> VQEGQKIDLPKKRYYRQRAHSNPFSDHQLEYPVSPQDMDWSKLYPYYKNAENGQMTKKVTIADIGCGFGGLMIDLSPAFPED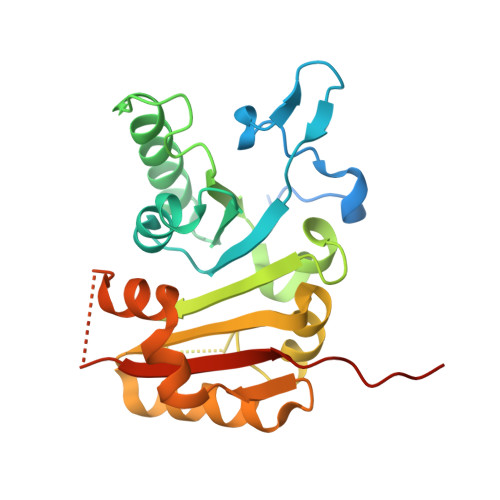LILGMEIRVQVTNYVEDRIIALRNNTASKHGFQNINVLRGNAMKFLPNFFEKGQLSKMFFCFPDPHFKQRKHKARIITNTLLSEYAYVLKEGGVVYTITDVKDLHEWMVKHLEEHPLFERLSKEWEENDECVKIMRNATEEGKKVERKKGDKFVACFTRLPTPAILHHHHHH>QTNANDLRNNEVFFISPSNNTNKVLDKISQSEVKLWNKLSGANQKWRLIYDTNKQAYKIKVMDNTSLILTWNAPLSSVSVKTDTNGDNQYWYLLQNYISRNVIIRNYMNPNLVLQYNIDDTLMVSTQTSSSNQFFKFSNCIYESFNNSTCKIQTSLTIKFIDKNQNSNNVTIWSWNNGDNQKWKILYNESKMAYTLTCIKNNEYLTWFSSIGNNVGTYRTEGNNDQYWFINYLNNDASMYTISNFSNQSKFLDVVNSGLADGTNVQVWDSNGTSAQKWI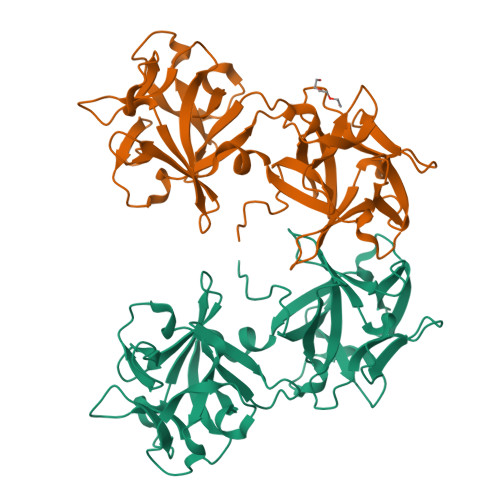ITRL[2x]>[2x]GGPAPLSTMQ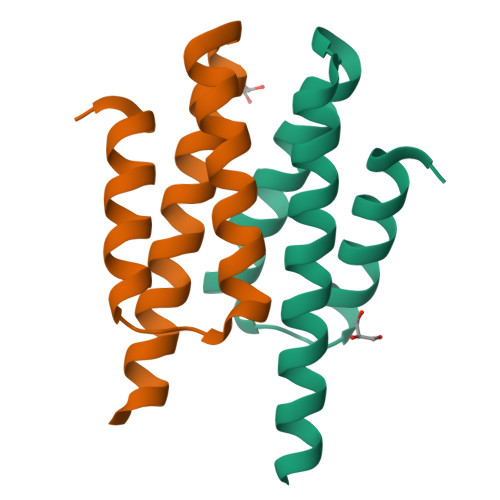TALMRLRTYHPSPIILKPVEQAVNHAITLVNTSPSSVVDALCRSLAELCLGLVQEAIDASILSQQESSNSLDLVRHTP[4-[[5-chloranyl-4-(methylamino)-7~{H}-pyrrolo[2,3-d]pyrimidin-2-yl]amino]-3-methoxy-phenyl]-morpholin-4-yl-methanone 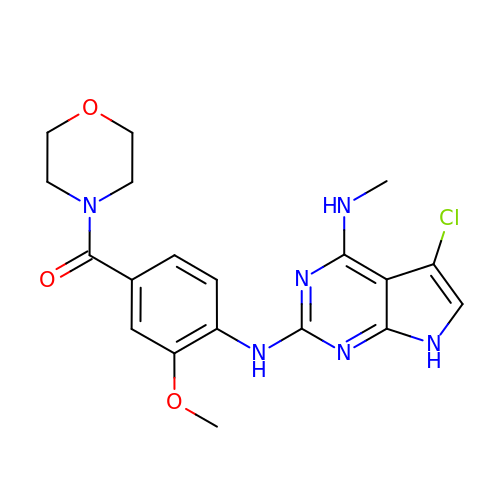| C19 H21 Cl N6 O3 | HUEKBQXFNHWTQQ-UHFFFAOYSA-N{[6-(4-methylphenyl)thieno[2,3-d]pyrimidin-5-yl]methyl}phosphonic 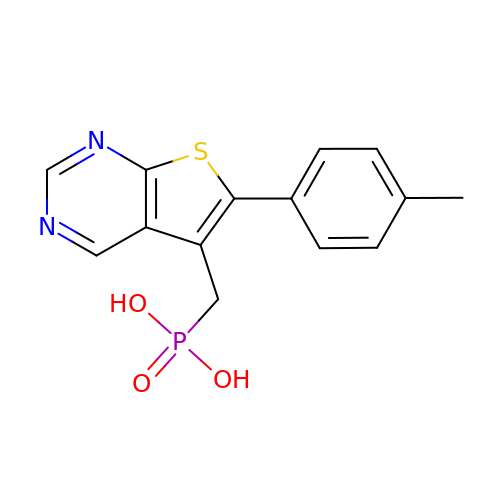acid | C14 H13 N2 O3 P S | YOCFRXSVLBRCJU-UHFFFAOYSA-N> MCIGMDIRDFFAQSAGRWFSQRTSHH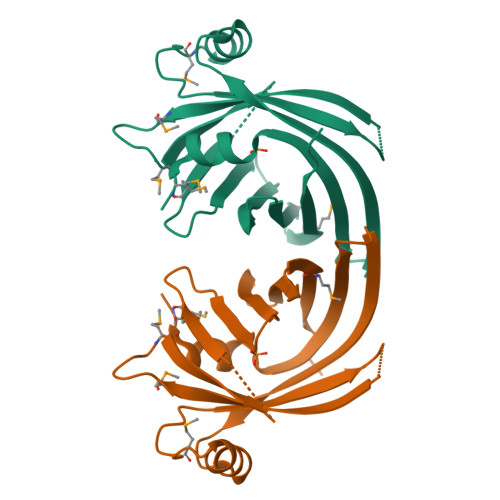LAFKQTESGKSQLTIELLSVDDPAVIALCQQYDMDPAWAVCGARVSWDGTMEWDNEKHEGSTVLVPIMDQGSRMEGKLLREMGYAEKAPVAGRFSMGSDGALTLITEYETIYSEERLWFASPNLRLRTSILKRFGGFSMASFCSEIRLGVTQPANSLEHHHHHH>[3x]GASTLTVHVRSEEWDLMTFDANPYDSVKKIKEHVRSKTKVPVQDQVLLLGSKILKPRRSLSSYGIDKEKTIHLTLKVVKPSDE

FAT10 is the only UBL modifier to directly target proteins for proteasomal degradation independently of Ub attachment. At the very C-terminus FAT10 carries a di-Gly motif that is a hallmark for the covalent attachment of Ub family modifiers to substrates through a conserved enzyme cascade. To characterize the structures of the FAT10 domains in more detail, we crystallized the N-domain and solved the solution NMR structure of the C-domain, since we could not obtain crystals of the latter. Both domains adopt the typical ββαββαβ β-grasp UBL fold.

To improve the long-term stability of the wild-type (WT) human FAT10 protein, we replaced the four cysteines in FAT10 with Ser, Thr, or Leu depending on whether they were predicted by bioinformatics analysis to be solvent-exposed or buried (C7T and C9T in the N-domain; C134L and C162S in the C-domain). For further structural studies, we designed a Cys-free FAT10 construct lacking the N-terminal four residues (ΔN FAT10; amino acids 5–165) and Cys-free constructs of the individual N- and C-terminal domains (amino acids 5–86 and amino acids 85–165, respectively; hereafter referred to as N- and C-domain). The N-domain crystallized readily and we solved its structure at 1.95 Å resolution by molecular replacement. We could resolve three virtually identical protein chains in the asymmetric unit that superimposed with a backbone root mean square deviation (r.m.s.d.) of 0.66 ± 0.01 Å for amino acids 8–81. Only the N- and C-terminal residues (amino acids 6–7 and 82–84, respectively) display distinct conformations and increased B factors showing that these residues are disordered and not part of the UBL fold. Of note, the side chains of residues 7 and 9 that are cysteines in the native human FAT10 sequence are indeed solvent exposed and only residue 9 is part of the UBL fold. As in Ub, the core of the UBL fold is stabilized by a dense hydrophobic interaction network that is almost void of aromatic residues. Overall, comparison of the FAT10 N-domain structure with Ub showed that not only the structured regions are well-conserved, but also the lengths of the loops except for the α2–β5 loop that contains two additional residues in the N-domain. Interestingly, the hydrophobic patch in Ub (L8, I44, and V70) that is used for most Ub–protein interactions, is neither conserved in the FAT10 N-domain (E15, L51, and K79) nor in the C-domain (S95, T133, and A159). To compare the FAT10 N- and C-domains in more detail and to identify conserved regions, we generated a multiple sequence alignment of FAT10 proteins. This revealed a conserved surface in the FAT10 N-domain that mainly consisted of the β5 strand.>MTTAGVSRRPGRLAGKAAIVTGAAGGIGRATVEAYLREGASVVAMDLAPRLAATRYEEPGAIPIACDLADRAAIDAAMADAVARLGGLDILVAGGALKGGTGNFLDLSDADWDRYVDVNMTGTFLTCRAGARAMVAAGAGKD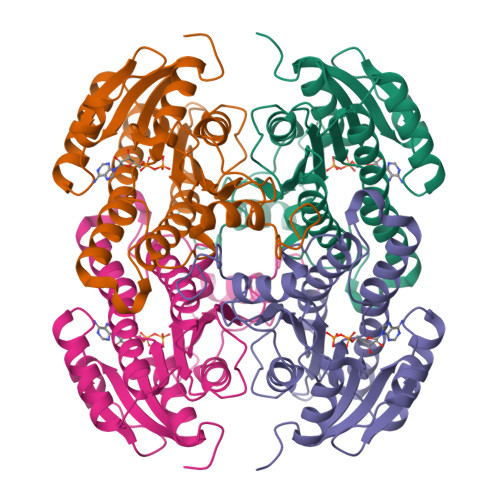GRSARIITIGSVNSFMAEPEAAAYVAAKGGVAMLTRAMAVDLARHGILVNMIAPGPVDVTGNNTGYSEPRLAEQVLDEVALGRPGLPEEVATAAVFLAEDGSSFITGSTITIDGGLSAMIFGGMREGRR[8x]N-(3-METHYLBUT-2-EN-1-YL)-9H-PURIN-6-AMINE 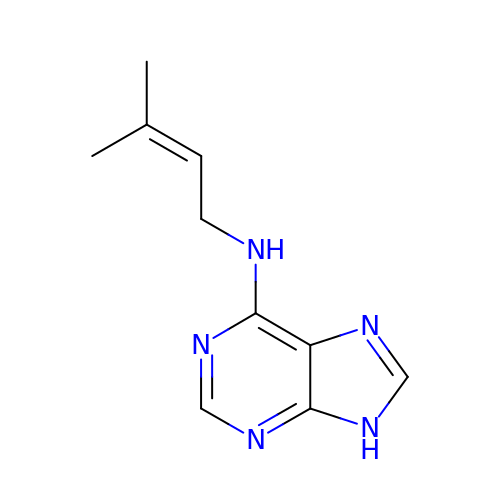| C10 H13 N5 | HYVABZIGRDEKCD-UHFFFAOYSA-N>[4x]MAPTVKLKPYCQNIADAATIDSTQYPPEVVRKAEAASIIDDPKALEGLPDVYLEEKTINRKNGSKIELTITRPLDTENQVLPPIVFFHGGGWVVGSKLTHRRTVYELTVRARAAVIFVNYSLSPEVRFPTALEECLDAVVWVAKEENAKSINVDPTKLVVAGDSAGGNLSAVVCIRAKQLGLNIIKGQVLIYPVTDDNFETDSYKQFAENYYLTRKLMVWFFDHYIPDKKDRQSIFACPLKASIDD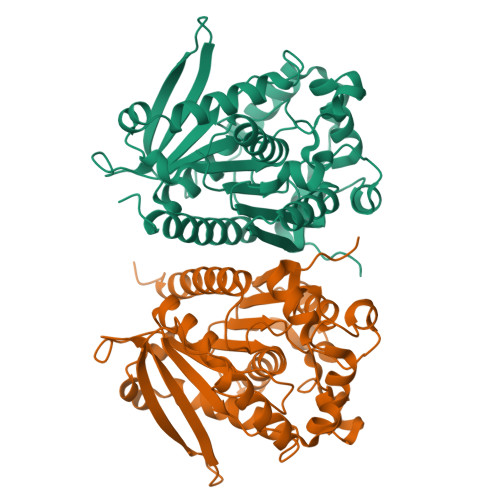LRVLPRALVITAEADVLREEGEAYARKLIEAGNDVTAVRYLGIIHGIFNLATLSPTGSEILDHIVAWLQKTWKLEHHHHHH>SAKDERAREILRGFKLNWMNLRDAATGKILWQGTEDLSVPGVEHEARVPKKILKCKAVSRELNFSSTEQMEKFRLEQKVYFKGQCLEEWFFEFGFVIP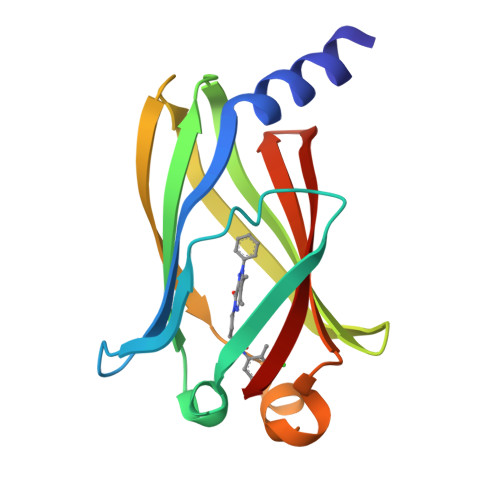NSTNTWQSLIEAAPESQMMPASVLTGNVIIETKFFDDDLLVSTSRVRLFYV[2x]>[6x]AKVF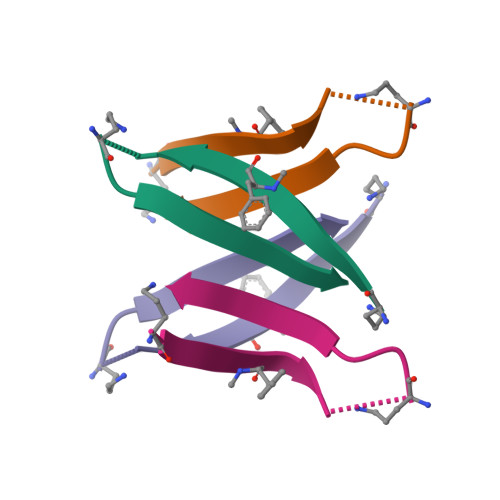FAADAAIIGLMV>[2x]QGPSSP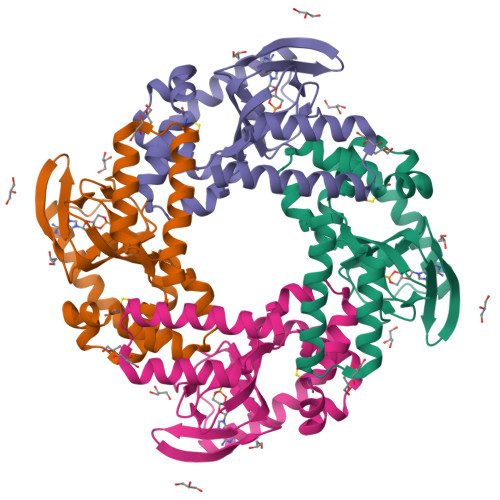MDSSRRQYQEKYKQVEQYMSFHKLPPDTRQRIHDYYEHRYQGKMFDEESILGELSEPLREEIINFNCRKLVASMPLFANADPNFVTSMLTKLRFEVFQPGDYIIREGTIGKKMYFIQHGVVSVLTKGNKETKLADGSYFGEICLLTRGRRTASVRADTYCRLYSLSVDNFNEVLEEYPMMRRAFETVALDRLDRIGKKNSILLH> M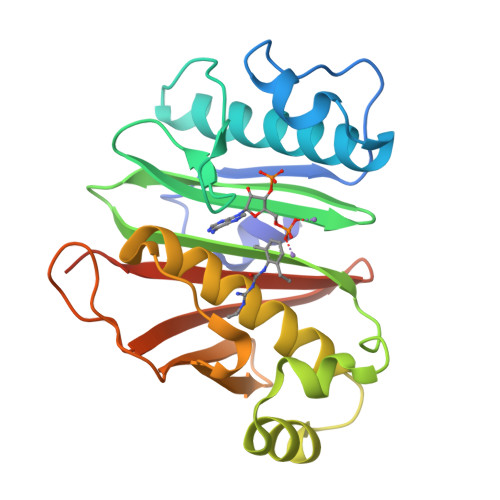PVTDQLIASVVPELLPSAELYEDPPGLEPLPEEEPLIAKSVAKRRNEFITVRYCARQALSVLGIPEVPILKGDKGQPLWPDGIVGSMTHTEGFRGAVVGRTGEVRSVGIDAEPHDVLPNGVLKSIALPVERDELDALPAGTHWDRLLFCAKETTYKAWFPLTARWLGFEDAHITIDPDGTFTSRILVDGRANDGTVLSAFDGRWIIDKGLILTAIVVPKLAAALEHHHHHH(3R)-4,4-DIFLUORO-3-[(4-METHOXYPHENYL)SULFONYL]BUTANOIC ACID | C11 H12 F2 O5 S | 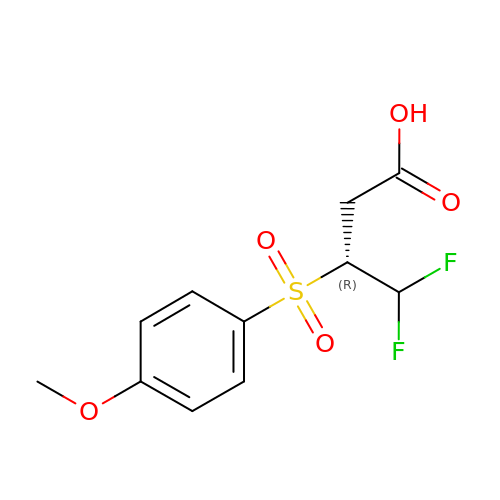OBQLOVWIRUXBAW-SECBINFHSA-N Na+/H+ exchangers (NHEs) are ancient membrane‐bound nanomachines that work to regulate intracellular pH, sodium levels and cell volume. Here, we report the cryogenic electron microscopy structure of NHE isoform 9 (SLC9A9) from Equus caballus at 3.2 Å resolution, an endosomal isoform highly expressed in the brain and associated with autism spectrum (ASD) and attention deficit hyperactivity (ADHD) disorders. Despite low sequence identity, the NHE9 architecture and ion‐binding site are remarkably similar to distantly related bacterial Na+/H+ antiporters with 13 transmembrane segments. The NHE9 monomer consists of 13 TMs with an extracellular N‐terminus and intracellular C‐terminus.

NHE9* sample preparation was optimized for grid preparation, cryo‐EM data acquisition and structural determination at an active pH of 7.5. We combined 3D classes from two independent data collections of ~ 1.4 million particles, from which an EM map was reconstructed to 3.5 Å according to the gold‐standard Fourier shell correlation (FSC) 0.143 criterion, which used ~ 5% of the total collected particles. The EM maps were well resolved for the TMs, but a few of the connecting loop residues and a larger, extracellular loop of 52 residues, located between TM2 and TM3, could not be built (Fig EV2A). Surprisingly, there was no obvious density for any of the 90‐residue long C‐terminal tail regulatory domain (CTD), likely a result of its predicted dynamics and intrinsic disorder (Fig EV2A; Norholm et al, 2011; Hendus‐Altenburger et al, 2014; Pedersen & Counillon, 2019). The NHE9* construct contains 97 residues of the C‐terminal regulatory domain (blue‐dotted circle), but no corresponding additional density was apparent as compared to the NHE9 ΔCTD density maps. Despite extensive efforts, we were unable to obtain any structural information for the regulatory domain of NHE9. It, therefore, seems unlikely that the C‐terminal tail in NHE9 interacts tightly with the transporter module in the absence of binding partners. As model building revealed only minor differences between NHE9* and NHE9 ΔCTD structures, the later was used for all subsequent analysis due to its moderately better resolution (Fig EV2C). Superimposition of NHE9* (wheat) and NHE9 ΔCTD (core transport domains (blue), dimerization domains (orange), linker helices (grey)) structures, which show only small differences in the most mobile regions.

>GAVELLVFNFLLILTILTIWLFKNHRFRFLHETGGAMVYGLIMGLILRYATAPTDIESGTVYDCGKLAFSPSTLLINITDQVYEYKYKREISQHNINPHLGNAILEKMTFDPEIFFNVLLPPIIFHAGYSLKKRHFFQNLGSILTYAFLGTAISCIVIGLIMYGFVKAMVYAGQLKNGDFHFTDCLFFGSLMSATDPVTVLAIFHELHVDPDLYTLLFGESVLNDAVAIVLTYSISIYSPKENPNAFDAAAFFQSVGNFLGIFAGSFAMGSAYAVVTALLTKFTKLCEFPMLETGLFFLLSWSAFLSAEAAGLTGIVAVLFCGVTQAHYTYNNLSLDSKMRTKQLFEFMNFLAENVIFCYMGLALFTFQNHIFNALFILGAFLAIFVARACNIYPLSFLLNLGRKHKIPWNFQHMMMFSGLRGAIAFALAIRDTESQPKQMMFSTTLLLVFFTVWVFGGGTTPMLTWLQI[2x]>MPYKNILTLISVNNDNFENYFRKIFLD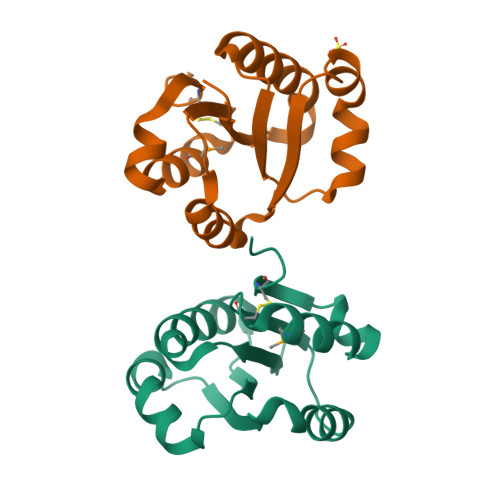VRSSGSKKTTINVFTEIQYQELVTLIREALLENIDIGYELFLWKKNEVDIFLKNLEKSEVDGLLVYCDDENKVFMSKIVDNLPTAIKRNLIKDFCRKLS[2x]>GPLGSSGNLLQVLMSFPSLTN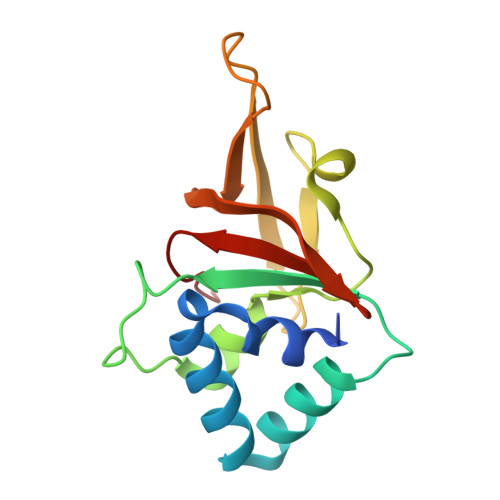FLTEVLAYSNSSARGRAFLEHLTDLSIRGTLFVPQNSGLGENETLSGRDIEHHLANVSMFFYNDLVNGTTLQTRVGSKLLITASQDPLQPTETRFVDGRAILQWDIFASNGIIHVISRPLKAP[2x]> SMAEVTIPIIVKDTTSFYWQIVLAGARKAGKDLGVKVPELGAQAETDVNGQISILENAVAGKPAAIVISPTEFKALGKPVDEAAKSVPIIGIDSGADS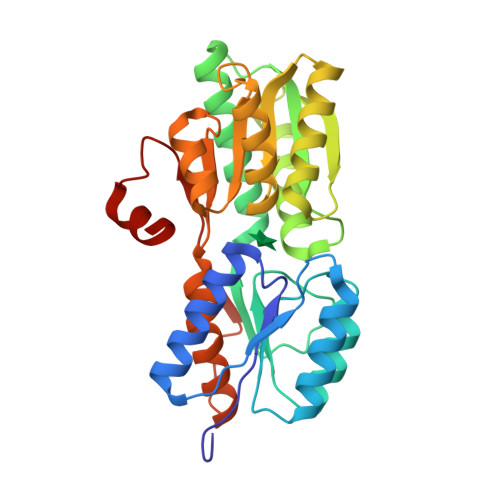KAFKSFLTTDNTQGGRIAADGLAAAIKAMTGKEEGDVVIITNTPGAGSLEQRRTGFLDQVKTKYPGLKVVADKYADGQATTGLNIMTDLITANPKIVGVFASNLIMAQGVGQAIAENKLSDKVKVIGFDSDDKTLGFLKSGAIAGLVVQDPYRMGYDGIKTALAVSKGEKVEANVDTGANLVTKANMSDPKIEALINPKVK>MSSILPFTPPIVKRLLGWKKGEQNGQEEKWCEKAVKSLVKKLKKTGQLDELEKAITTQNVNTKCITIPRSLDGRLQVSHRKGLPHVIYCRLWRWPDLHSHHELRAMELCEFAFNMKKDE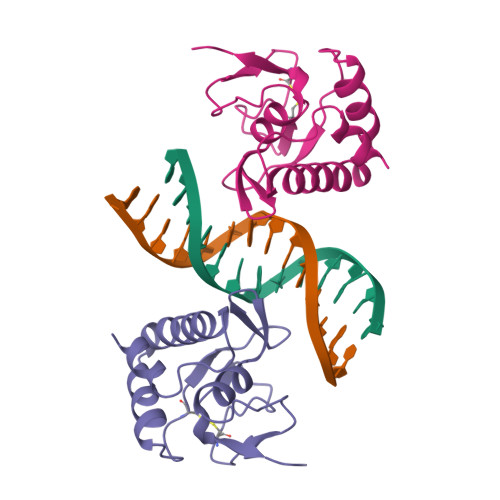VCVNPYHYQRVET[2x]> MEHHHHHHMPVFHTRTIESILEPVAQQISHLVIMHEEGEVDGKAIPDLTAPVAAVQAAVSNLVRVGKETVQTTEDQILKRDMPPAFIKVENACTKLVQAAQMLQSDPYSVPARDYLIDGSRGILSGTSDLLLTFDEAEVRKIIRVCKGILEYLTVAEVVETMEDLVTYTKNLG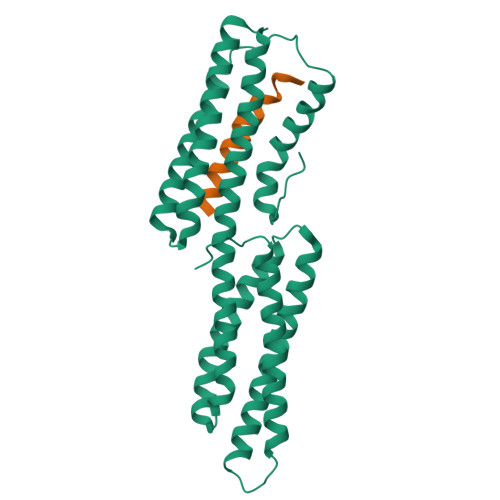PGMTKMAKMIDERQQELTHQEHRVMLVNSMNTVKELLPVLISAMKIFVTTKNSKNQGIEEALKNRNFTVEKMSAEINEIIRVLQLTSWDEDAW;> NNDITAENNNIYKAAKDVTTSLSKVLKNIN>[3x]MPLGLLWLGLALLGALHAQAQDSTSDLIPAPPLSKVPLQQNFQDNQFQGKWYVVGLAGNAILREDK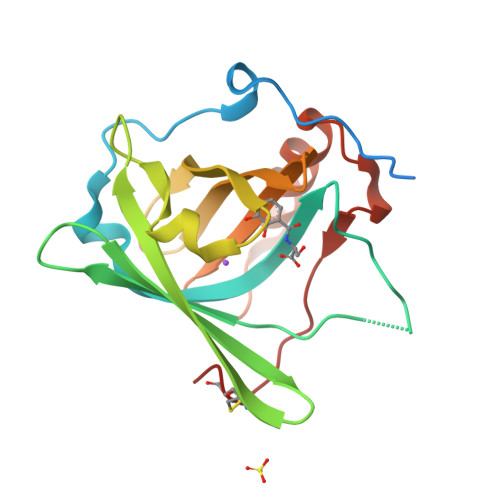DPQKMYATIYELKEDKSYNVTSVLFRKKKCDYWIRTFVPGSQPGEFTLGNIKSYPGLTSFLVRVVSTNYNQHAMVFFKKVSQNREYFKITLYGRTKELTSELKENFIRFSKSLGLPENHIVFPVPIDQCIDG>GEGMWVPQQLPEIAGPLKKAGLKLSPQQISDLTGDPMGAVVALGGCTASFVSPNGLVVTNHACAYGAIQLNSTAENNLIKNGFNAPTTADEVSAGPNARVFVLDEITDVTKDAKAAIAAAGDDALARTKALEAFEKKLIADCEAEAGFRCRLYSFSGGNTYRLFKNLEIKDVRLAYAPPGSVGKFGGDIDNWMWPRHTGAFAFYRAYVGKDGKPAAFSKDNVPYQPKHWLKFADQPLGAGDFVMVAGYPGSTNRYALAAEFDNTAQWTYPTIARHYKNQIAMVEAAGKQNADIQVKYAATMAGWNNTSKNYDGQLEGFKRIDAAGQKLREEAAVLGWLKGQGAKGQPALDAHAKLLDLLEQSKATRDRDLTLALFNNTAMLGSATQLYRLSIEREKPNAERESGYQERDLPAIEGGLKQLERRYVAAMDRQLQEYWLNEYIKLPADQRVAAVDAWLGGNDAAAVKRALDRLAGTKLGSTEERLKWFAADRKAFEASNDPAIQYAVAVMPTLLKLEQERKTRAGENLAARPVYLQALADYKKSQGEFVYPDANLSLRITFGNVMGYAPKDGMEYTPFTTLEGVVAKETGQDPFDSPKALLDAVAAKRYGGLEDKRIGSVPVNYLSDLDITGGNAGSPVLDAHGKLVGLAFD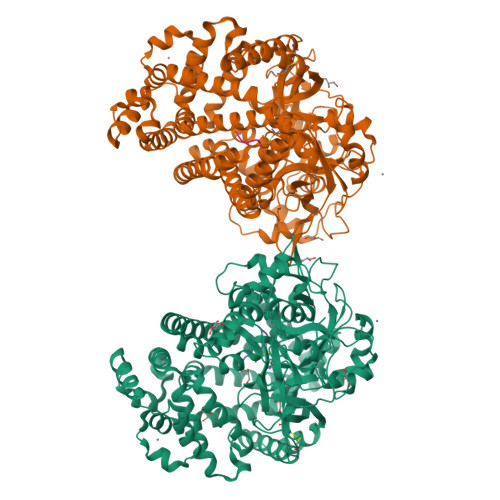GNWESVSSNWVFDPKMTRMIAVDGRYLRWIMQEVYPAPQLLKEMNVGK[2x];>[2x]DRVYIHPF Apical Membrane Antigen 1 (AMA1), a type 1 transmembrane protein of the Plasmodium parasite, includes an ectodomain, a transmembrane region and a cytoplasmic domain. The ectodomain comprises three domains referred to as Domain 1, Domain 2 and Domain 3. AMA1 is produced in the microneme organelles and transferred to the parasite surface just prior to or during red blood cell (RBC) invasion. AMA1 appears to be essential for invasion since, for several Plasmodium species, antibodies raised against the ectoplasmic region of the protein have been shown to inhibit invasion, and immunization with AMA1 in animal models protects against infection.

The free PkAMA1 protein crystallized in space group C2 with two molecules (A and B) in the asymmetric unit and the structure was refined at 2.45 Å resolution. The polypeptide chain of molecule A was traced from Ser52 to Glu397 (thus including eight residues of the c-myc tag), with main-chain gaps Ala131-Asp132, Ser212-Lys215 and Gly328-Asn331 due to conformational mobility. Molecule B was built from Ser52 to Asp398 with main-chain gaps Ser212-Ala217 and Gly328-Ser332. The two molecules are very similar, with an r.m.s.d. of 0.34 Å in Cα positions over the 332 common residues in the PkAMA1 sequence. The D2 loop of PkAMA1, which is displaced upon binding of the RON2 component of the RON receptor complex in the homologues TgAMA1 and PfAMA1, could be completely traced in both molecules except for the short region Gly328-Ser332. Nonetheless, the high temperature factors of this region indicate a propensity to structural mobility. Interestingly, the D2 loop adopts a different conformation in PkAMA1 to that which has been observed in PfAMA1. This could be due to sequence differences between the two homologues or could arise from inherent flexibility in this region of AMA1.

>EFPIIERSIRMSNPWKAFMEKYDLERAHNSGIRIDLGEDAEVGNSKYRIPAGKCPVFGKGIVIENSKVSFLTPVATGAQRLKEGGFAFPNADDHISPITIANLKERYKENADLMKLNDIALCKTHAASFVIAEDQNTNYRHPAVYDEKEKTCYMLYLSAQENMGPRYCSPDSQNKDAMFCFKPDKNEKFDNLVYLSKNVRNDWENKCPRKNLGNAKFGLWVDGNCEEIPYVNEVEARSLRECNRIVFEASASDQPRQYEEELTDYEKIQEGFRQNNRDMIKSAFLPVGAFNSDNFKSKGRGYNWANFDSVNNKCYIFNTKPTCLINDKNFFATTALSHPQEVDNEFPGLEQKLISEEDLNSAVDHHHHHH[2x]> A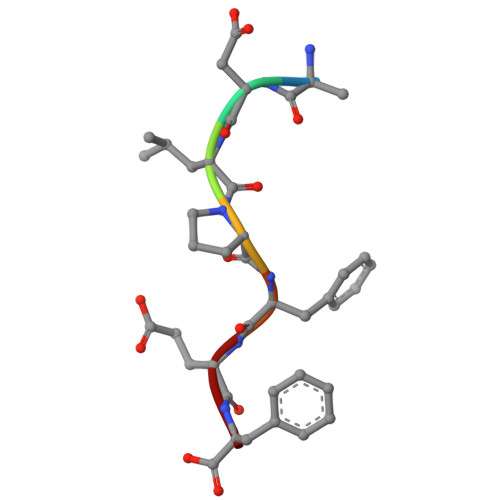DLPFEF> ESAFNQTEFNKLLLECVVKTQSSVAKILGILSLS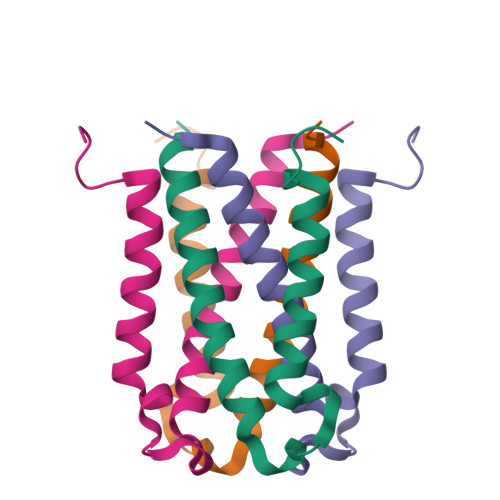PHVSGNSKFEYANMVEDIREKVSSEMERFFPKNDDE> TRDQNGTWEMESNENFEGYMKALDIDFATRKIAVRLTQTLVIDQDGDNFKWKTTSTFRNYDVDFTVGVEFDEYTKSLDNRHVKALVTWEGDVLVCVQKGEKENRGWKKW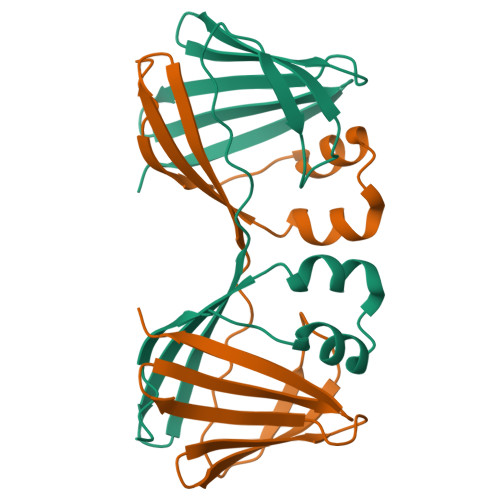IEGDKLYLELTCGDQVCRQVFKKK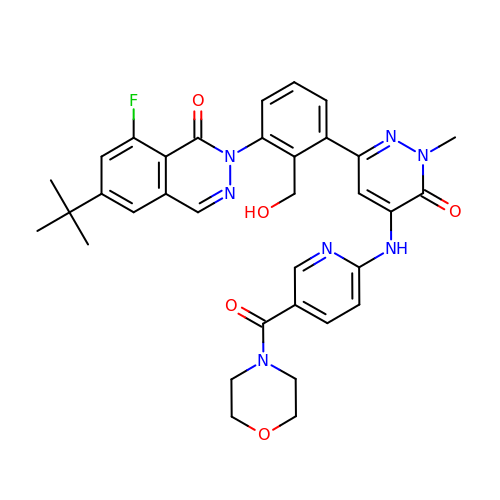6-~{tert}-butyl-8-fluoranyl-2-[2-(hydroxymethyl)-3-[1-methyl-5-[(5-morpholin-4-ylcarbonylpyridin-2-yl)amino]-6-oxidanylidene-pyridazin-3-yl]phenyl]phthalazin-1-one | C34 H34 F N7 O5 | GLLQSOROVXWYRC-UHFFFAOYSA-N> MIH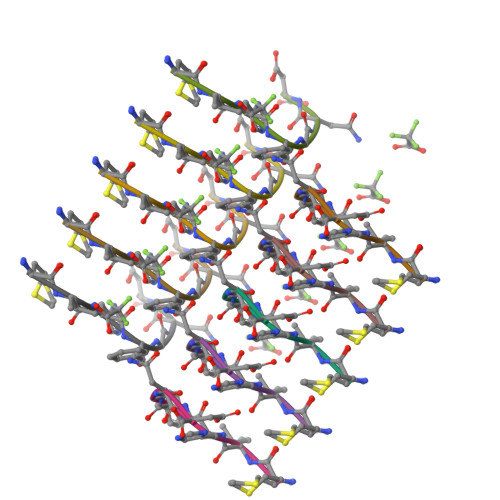FGND> KETAAAKFERQHMDSSTSAASSSNYCNQMMKSR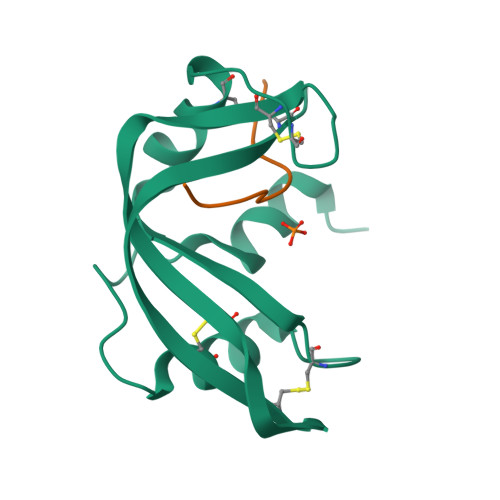NLTKDRCKPVNTFVHESLADVQAVCSQKNVACKNGQTNCYQSYSTMSITDCRETGSSKYPNCAYKTTQANKHIIVACEG;> PYVPVHFDASV2′,3′-cyclic nucleotide 3′-phosphodiesterase (CNPase) comprises 4% of total myelin protein in the central nervous system (CNS), being the most abundant CNS non-compact myelin protein4. CNPase consists of an N-terminal polynucleotide kinase-like domain10, a catalytic phosphodiesterase domain11, and a membrane-anchored C-terminal tail, which contains a cysteine residue that undergoes isoprenylation. The catalytic domain enables the rapid hydrolysis of nucleoside 2′,3′-cyclic phosphates to nucleoside 2′-phosphates. The CNPase catalytic site, lying in a groove between two lobes, has pseudo two-fold symmetry and contains two apposing His-X-Thr-X (X denotes a hydrophobic residue) motifs, characteristic for 2H phosphoesterases 113537.

Pro225 and Pro296 reside in loops α3-β2 and α6-β5, respectively, flanking the edges of the active site – Pro296 near the adenine moiety and Pro225 on the 5′-side of the ligand, next to Pro226. The kcat values of P225G and P296G are slightly higher compared to the wild type enzyme, most likely due to conformational flexibility offered by the glycine residues. P225G is the only mutant with an increased specificity constant (kcat/KM). We attempted to co-crystallize P225G in the presence of ligands. However, the reasonably low resolution (2.70 Å) crystal structure, which we obtained from crystals grown in the presence of reduced nicotinamide adenine dinucleotide 2′,3′-cyclic phosphate (2′,3′-cNADP+), contains only poorly defined ligand density in the active site.

> GLEKDFLPLYFGWFLTKKSSETLRKAGQVFLEELGNHKAFKKELRHFISGDEPKEKLELVSYFGKRGPGVLHCTTKFCDYGKAAGAEEYAQQEVVKRSYGKAFKLSISALFVTPKTAGAQVVLTDQELQLWPSDLDKPSASEGLPPGSRAHVTLGCAADVQPVQTGLDLLDILQQVKGGSQGEAVGELPRGKLYSLGKGRWMLSLTKKMEVKAIFTGYYG>GGGRELPTLLSLLLEALSCPDSVVQLSTLSCLQPLLLEAPQIMSLHVDTLVTKFLNLSSSYSMAVRIAALQCMHALTRLPTSVLLPYKSQVIRALAKPLDDKKRLVRKEAVSARGEWFLLGSPGS[2x];>GGGRPTEIENINPNVYDRIKERVLTANEEDENVPDPFDKREIFDLIRNINDPEHPLTLEELHVVQEDLIRINDSQNSVHISFTPTIPHCSMATLIGLSIRVKLLRSLPPRFKVTVEITPGTHASELAVNKQLADKERVAAALENNHLAEVINQCIAAKG[2x];>[2x]GGGRGRLILEHTLQGHKGRIWGVAWHPKGNVFASCGEDKAIRIWSLTGNTWSTKTILSDGHKRTIREIRWSPCGQYLASASFDATTAIWSKSSGEFECNATLEGHENEVKSVSWSRSGGLLATCSRDKSVWIWEVAGDDEFECAAVLNPHTQDVKRVVWHPTKDILASASYDNTIKMFAEEPIDNDWDCTATLTSHTSTVWGIDFDADGERLVSCSDDTTIKIWRAYHPGNTAGVATPDQQTVWKCVCTVSGQHSRAIYDVSWCKLTGLIATACGDDGIRIFKESSDSKPDEPTFEQITAEEGAHDQDVNSVQWNPV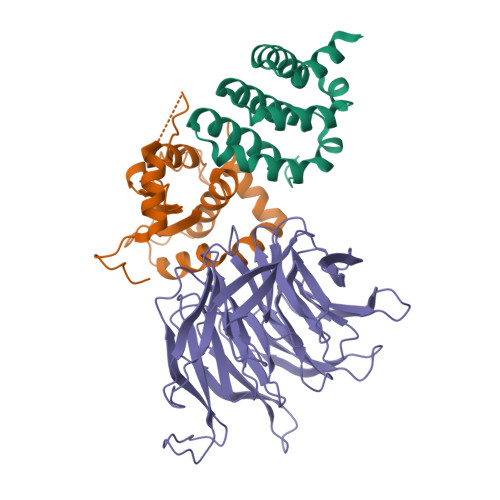VAGQLISCSDDGTIKIWKVTE We report here structure-function studies of soluble periplasmic LT of Campylobacter jejuni. The LT Cj0843 was identified from a virulent strain of C. jejuni and localized in the periplasm. The LT enzymes cleave the PG MurNAc-GlcNAc glycosidic bond similar to lysozyme with the noted difference that LTs have an additional (2nd) cyclization step; this step requires a boat conformation of MurNAc leading to a 1,6-anhydromuramyl product as the predominant terminal saccharide moiety. The crystal structure of the soluble LT Cj0843 from C. jejuni revealed an unusual doughnut-shaped structure containing four domains: NU-, U-, L-, and C-domains.

The structures from both crystal forms are very similar with a root-mean-square-deviation (RMSD) for 509 Cα atoms of 0.75 Å. At the N-terminus is a small helical domain (NU-domain) connected via a flexible linker to the helical U-domain. This flexible linker (residues 75–83) is partially resolved in the P3121 crystal form and fully resolved in the I23 crystal form; it spans 22Å between ordered anchor points I74 and Y84 in the NU-domain and U-domain, respectively. The most prominent feature of the electrostatic potential surface of Cj0843 is its predominantly positively charged inner ring surface. The outer ring surface of these ring-shaped proteins shows a more random distribution of positive, negative, and neutral residues. This ensemble of positive charges on the inside of the ring of Cj0843 explains why the majority of sulfate and acetate ions, that co-crystallized at 200mM concentration in both crystal forms, were observed along the inner ring of the doughnut-shaped Cj0843 protein.

> MQYSIEKLKKEENSLAKDYYIYRLLEKNKISKKDAQDLNSHIFRYIGKIKSELEKIIPLKPYINPKYAKCYTYTANTILDANLTCQSVRLNSLVFIASLNSKDRTTLAQTFKNQRPDLTNLLLAFNTSDPMSYIVQKEDINGFFKLYNYSKKYDLDLNTSLVNKLPNHIGFKDFAQNIIIKKENPKFRHSMLEINPENVSEDSAFYLGVNALTYDKTELAYDFFKKAAQSFKSQSNKDNAIFWMWLIKNNEEDLKTLSQSSSLNIYSLYAKELTNTPFPKIESLNPSKKKNNFNMQDPFAWQKINKQIRDANASQLDVLAKEFDTQETLPIYAYILERKNNFKKHYFIMPYYDNIKDYNKTRQALILAIARQESRFIPTAISVSYALGMMQFMPFLANHIGEKELKIPNFDQDFMFKPEIAYYFGNYHLNYLESRLKSPLFVAYAYNGGIGFTNRMLARNDMFKTGKFEPFLSMELVPYQESRIYGKKVLANYIVYRHLLNDSIKISDIFENLIQNKANDLNKS> ANTSSAYNSVYDFLRYHDRGDGLTVNGKTSYSIDQAAAQITRENVSWNGTNVFGKSANLTFKFLQSVSSIPSGDTGFVKFNAEQIEQAKLSLQSWSDVANLTFTEVTGNKSANITFGNYTRDASGNLDYGTQAYAYYPGNYQGAGSSWYNYNQSNIRNPGSEEYGRQTFTHEIGHALGLAHPGEYNAGEGDPSYNDAV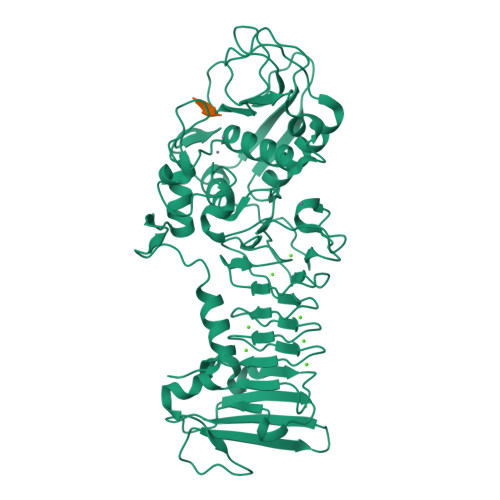YAEDSYQFSIHSYWGENETGADYNGHYGGAPMIDDIAAIQRLYGANMTTRTGDSVYGFNSNTDRDFYTATDSSKALIFSVWDAGGTDTFDFSGYSNNQRINLNEGSFSDVGGLKGNVSIAHGVTIENAIGGSGNDILVGNSADNILQGGAGNDVLYGGAGADTLYGGAGRDTFVYGSGQDSTVAAYDWIADFQKGIDKIDLSAFRNEGQLSFVQDQFTGKGQEVMLQWDAANSITNLWLHEAGHSSVDFLVRIVGQAAQSDIIV;> AKAA>MSDREFVTVDPVTIIIKECINLSTAMRKYSKFTSQSGVAALLGGGSEIFSNQDDYLAHTFNNLNTNKHNDPFLSGFIQLRLMLNKLKNLDNIDSLTILQPFLLIVSTSSISGYITSLALDSLQKFFTLNIINESSQNYIGAHRATVNALTHCRFEGSQQLSDDSVLLKVVFLLRSIVDSPYGDLLSNSIIYDVLQTILSLACNNRRSEVLRNAAQSTMIAVTVKIFSKLKTIEPVNVNQIYINDESYTNDVLKADTIGTNVESKEEGSQEDPIGMKVNNEEAISEDDGIEEEHIHSEKSTNGAEQLDIVQKTTRSNSRIQAYADDNYGLPVVRQYLNLLLSLIAPENELKHSYSTRIFGLELIQTALEISGDRLQLYPRLFTLISDPIFKSILFIIQNTTKLSLLQATLQLFTTLVVILGNNLQLQIELTLTRIFSILLDDGTANNSSSENKNKPSIIKELLIEQISILWTRSPSFFTSTFINFDCNLDRADVSINFLKALTKLALPESALTTTESVPPICLEGLVSLVDDMFDHMKDIDREEFGRQKNEMEILKKRDRKTEFIECTNAFNEKPKKGIPMLIEKGFIASDSDKDIAEFLFNNNNRMNKKTIGLLLCHPDKVSLLNEYIRLFDFSGLRVDEAIRILLTKFRLPGESQQIERIIEAFSSAYCENQDYDPSKISDNAEDDISTVQPDADSVFILSYSIIMLNTDLHNPQVKEHMSFEDYSGNLKGCCNHKDFPFWYLDRIYCSIRDKEIVMPEEHHGNEKWFEDAWNNLISSTTVITEIKKDTQSVMDKLTPLELLNFDRAIFKQVGPSIVSTLFNIYVVASDDHISTRMITSLDKCSYISAFFDFKDLFNDILNSIAKGTTLINSSHDDELSTLAFEYGPMPLVQIKFEDTNTEIPVSTDAVRFGRSFKGQLNTVVFFRIIRRNKDPKIFSKELWLNIVNIILTLYEDLILSPDIFPDLQKRLKLSNLPKPSPEISINKSKESKGLLSTFASYLKGDEEPTEEEIKSSKKAMECIKSSNIAASVFGNES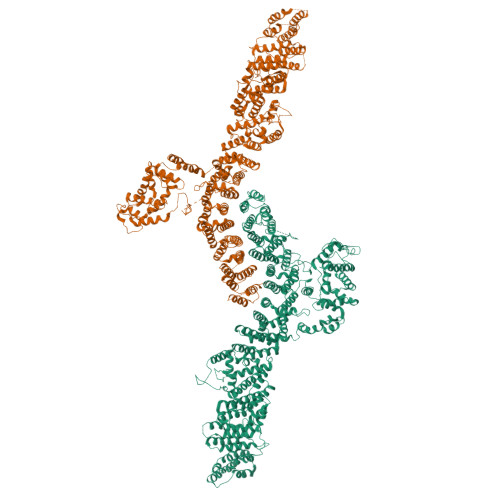NITADLIKTLLDSAKTEKNADNSRYFEAELLFIIELTIALFLFCKEEKELGKFILQKVFQLSHTKGLTKRTVRRMLTYKILLISLCADQTEYLSKLINDELLKKGDIFTQKFFATNQGKEFLKRLFSLTESEFYRGFLLGNENFWKFLRKVTAMKEQSESIFEYLNESIKTDSNILTNENFMWVLGLLDEISSMGAVGNHWEIEYKKLTESGHKIDKENPYKKSIELSLKSIQLTSHLLEDNNDLRKNEIFAIIQALAHQCINPCKQISEFAVVTLEQTLINKIEIPTNEMESVEELIEGGLLPLLNSSETQEDQKILISSILTIISNVYLHYLKLGKTSNETFLKILSIFNKFVEDSDIEKKLQQLILDKKSIEKGNGSSSHGSAHEQTPESNDVEIEATAPIDDNTDDDNKPKLSDVEKD[2x]> MARERIIGIPKLEDANDAGSKYSQECTLILTEGDSAKTSCLAGLSIVGRDKYGVFPLKGKLLNVRDASFKQLMDNKEIQNIFRIMGLDITDKNKDDIKGLRYGSLMIMTDQDYDGSHIKGLLINMIHKFWPSLLKHKGFLS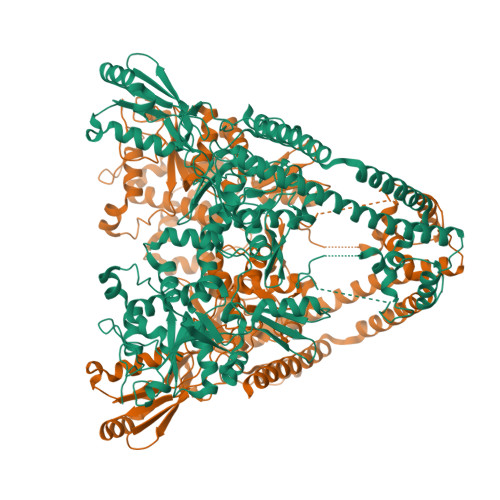EFVTPIVKVQKGSQEYSFFTIAEYEQWKENTNLLGWKIKYYKGLGTSTDREFKQYFSDIKNHKIMFLWTGDRDGDSIDMAFSKKRIEDRKLWLQNFILGSYVDHKEKDLSYYDFVNKELIYYSRYDTERSIPNIMDGWKPGQRKVLYGCFKRNLRNECKVAQLVGYIAEHSAYHHGESSLQQTIINMAQTFVGSNNINFLEPCGQFGSRKEGGKDASAARYIFTKLASSTRSIFNEYDDPILKYLNEEGQKIEPQYYIPVIPTILVNGCEGIGTGYSSFIPNYNYKDIIDNIKRYINKEPLIPMVPWYKDFKGRIESNGKTGYETIGIINKIDNDTLEITELPIKKWTQDYKEFLEELLTDEKHQLILDYIDNSSHEDICFTIKMDPAKLQKAEEEGLEKVFKLKSTLTTTNMTLFDPNLKLQRYSTELDILKEFCYQRLKAYENRKSYLISKLEKEKRIISNKTKFILAIVNNELIVNKKKKKVLVEELYRKGYDPYKDINKIKKEEIFEQELLDAADNPEDNEEIIAGITVKDYDYLLSMPIFSLTLEKVEDLLTQLKEKERELEILRNITVETMWLKDIEKVEEAIEFQRNVELSNREESNHHHHHH>MLSTGTKSLDSLLGGGFAPGVLTQVYGPYASGKTTLALQTGLLSGKKVAYVDTEGGFSPERLVQMAETRGLNPEEALSRFILFTPSDFKEQRRVIGSLKKTVDSNFALVVVDSITAHYRAEENRSGLIAELSRQLQVLLWIARKHNIPVIVINQVHFDSRTEMTKPVAEQTLGYRCKDILRLDKLPKPGLRVAVLERHRFRPEGLMAYFRITERGIEDVE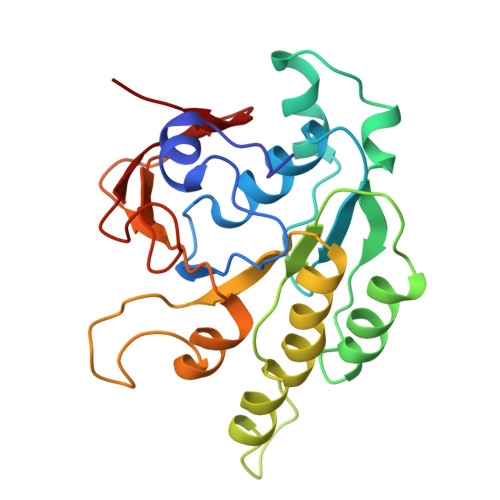[2x]GlgE is an α-maltose 1-phosphate:(1→4)-α-d-glucan 4-α-d-maltosyltransferase (starch synthase (maltosyl-transferring), EC 2.4.99.16) and a member of the carbohydrate-active enzymes database (CAZy) GH13_3 family. It is the third and defining enzyme of the four-step GlgE pathway that is responsible for the biosynthesis of a branched α-glucan. The key contribution that GlgE makes is to preferentially extend A chains, limiting the opportunity for GlgB to introduce a second branch into B and C chains. The enzyme consists of five domains, four of which are typical of the α-amylase family.

Co-crystallization and soaks of a different catalytically compromised E423A variant of GlgE, which lacks the acid/base catalytic side chain, were carried out with various substrates and/or substrate analogues. By using mutagenesis to prevent GlgE from slowly hydrolyzing malto-oligosaccharides, it was possible to obtain a structure with malto-octaose bound to the active site. The occupancy of the donor subsites −2 and −1 together with subsites +1 to +6 indicated that this represents a product-bound structure that reveals the locations of the first six acceptor subsites. An essentially identical structure was also obtained by soaking a crystal with maltoheptaose except that the +6 subsite was not occupied. This showed that it was possible to obtain a product-bound structure in the absence of a donor substrate analogue. The product-bound structures of the E423A variant of GlgE had an additional malto-oligosaccharide bound at a secondary site located on domain C. In each case, five glucose residues were well resolved, clearly showing that they that were wrapped around Tyr-646 of S. coelicolor GlgE. The non-reducing end of this malto-oligosaccharide occupied a pocket on the surface of the enzyme, precluding the ability to accommodate any more glucose residues at this location. By contrast, the reducing end glucose residue was flipped relative to the other residues such that its α-anomeric hydroxyl projected into solvent. The likelihood is that malto-octaose/maltoheptaose was bound to this site but that three/two glucose residues at the reducing end were not well ordered in the crystal.

>[2x]MPATHHSSATSAERPTVVGRIPVLDVRPVVQRGRRPAKAVTGESFEVSATVFREGHDAVGANVVLRDPRGRPGPWTPMRELAPGTDRWGATVTAGETGTWSYTVEAWGDPVTTWRHHARIKIPAGLDTDLVLEEGARLYERAAADVPGREDRRELLAAVDALRDESRPAASRLAAALTPQVDAVLARHPLRDLVTSSDPLPLLVERERALYGAWYEFFPRSEGTPHTPHGTFRTAARRLPAIAAMGFDVVYLPPIHPIGTTHRKGRNNTLSATGDDVGVPWAIGSPEGGHDSIHPALGTLDDFDHFVTEAGKLGLEIALDFALQCSPDHPWVHKHPEWFHHRPDGTIAHAENPPKKYQDIYPIAFDADPDGLATETVRILRHWMDHGVRIFRVDNPHTKPVAFWERVIADINGTDPDVIFLAAAFTRPAMMATLAQIGFQQSYTYFTWRNTKQELTEYLTELSGEAASYMRPNFFANTPDILHAYLQHGGRPAFEVRAVLAATLSPTWGIYSGYELCENTPLREGSEEYLDSEKYQLKPRDWTRAAREGTTIAPLVTRLNTIRRENPALRQLRDLHFHPTDKEEVIAYSKRQGSNTVLVVVNLDPRHTQEATVSLDMPQLGLDWHESVPVRDELTGETYHWGRANYVRLEPGRTPAHVCTVLRPSHPQIGGSHTT>MESKRNKPGKATGKGKPVGDKWLDDAGKDSGAPIPDRIADKLRDKEFKSFDDFRKAVWEEVSKDPELSKNL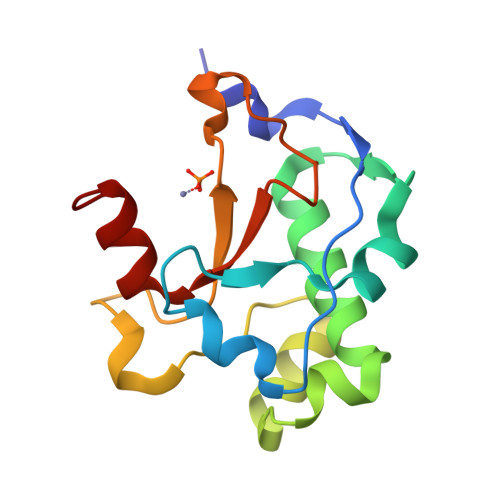NPSNKSSVSKGYSPFTPKNQQVGGRKVYELHHDKPISQGGEVYDMDNIRVTTPKRHIDIHRGK[4x]> KKPKNKDKDKKVPEPDNKKKKPKKEEEQKWKWWEEERYPEGIKWKFLEHKGPVFAPPYEPLPENVKFYYDGKVMKLSPKAEEVATFFAKMLDHEYTTKEIFRKNFFKDWRKEMTNEEKNIITNLSKCDFTQMSQYFKAQTEARKQMSKEEKLKIKEENEKLLKEYGFCIMDNHKERIANFK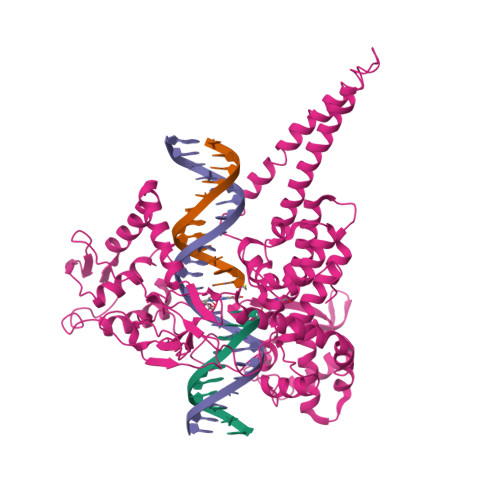IEPPGLFRGRGNHPKMGMLKRRIMPEDIIINCSKDAKVPSPPPGHKWKEVRHDNKVTWLVSWTENIQGSIKYIMLNPSSRIKGEKDWQKYETARRLKKCVDKIRNQYREDWKSKEMKVRQRAVALYFIDKLALRAGNEKEEGETADTVGCCSLRVEHINLHPELDGQEYVVEFDFLGKDSIRYYNKVPVEKRVFKNLQLFMENKQPEDDLFDRLNTGILNKHLQDLMEGLTAKVFRTYNASITLQQQLKELTAPDENIPAKILSYNRANRAVAILCNHQRAPPKTFEKSMMNLQTKIDAKKEQLADARRDLKSAKADAKVMKDAKTKKVVESKKKAVQRLEEQLMKLEVQATDREENKQIALGTSKLSYLDPRITVAWCKKWGVPIEKIYNKTQREKFAWAIDMADEDYEF> SMTPRNLAAWKISIPYVDFFEDPSSERKEKKERIPVFCIDVERNDRRAVGHEPEHW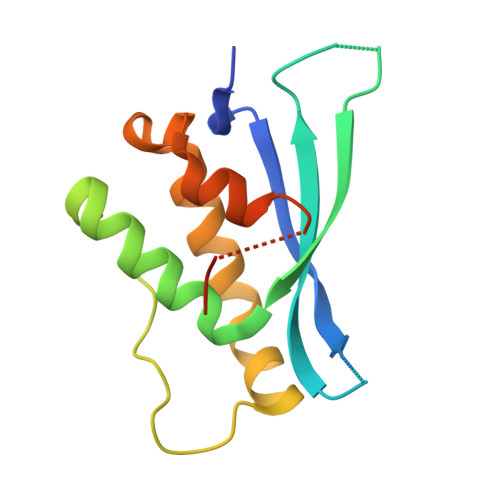SVYRRYLEFYVLESKLTEFHGAFPDAQLPSKRIIGPKNYEFLKSKREEFQEYLQKLLQHPELSNSQLLADFLSPNGGETQFLDKILPDVNL> APLVHHHHHHALANPAICRYPLGMSGGQIPDEDITASSQWSESTAAKYGRLDSEEGDGAWCPEIPVEPDDLKEFLQIDLHTLHFITLVGTQGRHAGGHGIEFAPMYKINYSRDGTRWISWRNRHG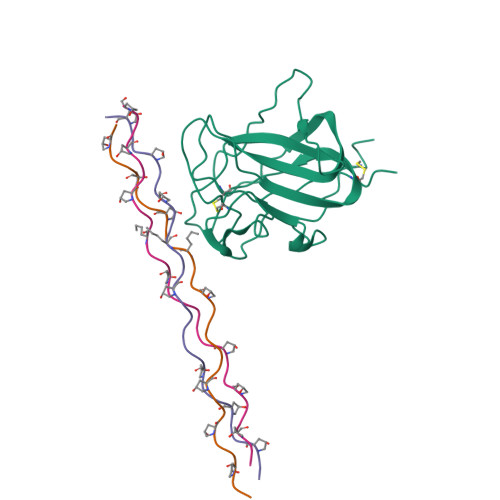KQVLDGNSNPYDIFLKDLEPPIVARFVRFIPVTDHSMNVCMRVELYGCVWLDG;>[3x]XGPPGPPGPPGPRGQPGVLGFPGPPGPPG> MGKRHRNLIDQITTWENLLDAYRKTSHGKRRTWGYLEFKEYDLANLLALQAELKAGNYERG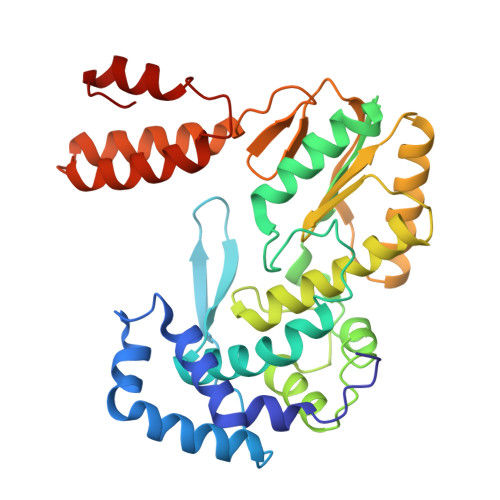PYREFLVYEPKPRLISALEFKDRLVQHALCNIVAPIFEAGLLPYTYACRPDKGTHAGVCHVQAELRRTRATHFLKSDFSKFFPSIDRAALYAMIDKKIHCAATRRLLRVVLPDEGVGIPIGSLTSQLFANVYGGAVDRLLHDELKQRHWARYMDDIVVLGDDPEELRAVFYRLRDFASERLGLKISHWQVAPVSRGINFLGYRIWPTHKLLRKSSVKRAKRKVANFIKHGEDESLQRFLASWSGHAQWADTHNLFTWMEEQYGIACH>[7x]MDKFRIMVQFLQANQESFMNGICGIMALASAQMYSSFEFTCPCLPDYNYAYGIGILIVPPIWFFLLGYVMNNNISVLTEEWKRPVGKRSKDPAVLRYMFSSMTQRALIAPAVWIAVTLMDGKSFLCAFSPTADLS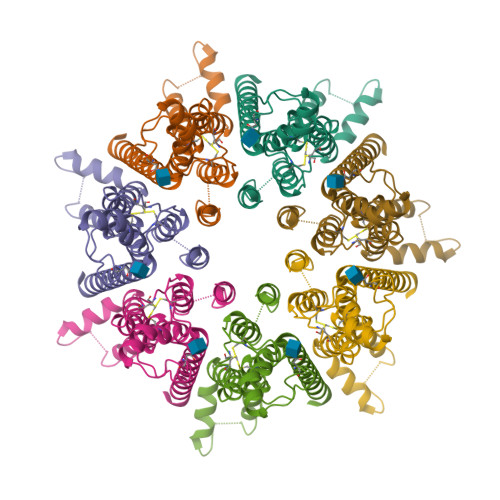EFVNESYQSLSQKELLKIQAKIPCKDIFEEHEIISREAATRYIRCLSQACGWTFLMVITLVAFLVRAIRPCFTQAAFLKTKYWSHYIDTERKLFDETCKEHAKSFAKVCIQQYFESISGEIVSQLPQSPAKKGKGNKDEDGEKQKSDEERLLGIRKEGDMNKVLWNWHTCKPPLLLSKRTEEMNGHAHLDTHSLTDERHTKKKAVVYYSKV> GRNRRRTVRSEGIDPEKAKLYQAPYFEKSEDEMNLITKLLTHNVLFSFLNTKDIKVVAGAMQRATFKHDDCIMEAGQTTCNKLYIIQSGHADIIKEGQKVYLKTEGTAVGELELMYDTPVVATVKVCTDELIAWVLDRDTYRNLVMGTAIRRRETYIQFLANVPFLGGLDSYEKLQLADALSSEEFSPGEYIIHYGEEGEWLYIIMEGTV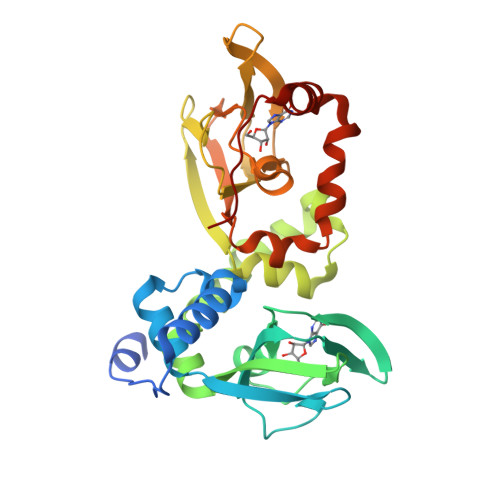EVIGRDADGEPTKVCEFTQGDHIGELEFLNNHRTVADVVATTHVITAKLNRRHFEMCLGPVIDVLKRCADDPKYEYYQNVLKTGAAQPSYVDDV>PLLERLKRRVVEGRKQGLEADLEEALKAGHKPLDLINGPLLAGMKEVGDLFGAGKMQLPFVLQAAEVMKRAVAYLEPHMEKKGEGKGTLVLATVKGDVHDIGKNLVDIILSNNGYRVVNLGIKVPIEEILKAVEAHKPHAVGMSGLLVKSTLVMKENLEYMRDRGYTLPVILGGAALTRSYVEELRAIYPNVYYAEDAFEGLRLMEELTGHAPPELTRKAPARPKREAPKVAPRARPVGEAPAVPRPPFFGVRVEEGLDLATIAHYVNKLALYRGQWGYSRKGLSREAWQALVEREAEPVFQRLLKEAMAEGWLEPKVLYGFFPVAREGEELLVFSPETGEVLERFRFPRQKGGGLSLVDYFRPRFAAPLGDEADWMPKEAFRAGARDVLGVQLVTMGEAPSRKAQALFASGAYQDYLFVHGFSVEMTEALAEYWHKRMRQMWGIAHQDATEIQKLFQQGYQGARYSFGYPACPDLADQAKLDRLMGFHRVGVRLTENFQLEPEHATSALVVHHPEARYFSVD[6x]

Cobalamin-dependent methionine synthase (MS) is a key enzyme in methionine and folate one-carbon metabolism. MS is a large multi-domain protein capable of binding and activating three substrates: homocysteine, folate, and S-adenosylmethionine for methylation. Achieving three chemically distinct methylations necessitates significant domain rearrangements to facilitate substrate access to the cobalamin cofactor at the right time. Here, we use a thermophilic MS homolog (tMS) as a functional MS model.

We selected cyanocobalamin (CN-Cbl), a stable and synthetic Cbl that does not support catalysis. To that end, apo-Cap:Cob:Act tMS crystals were soaked with CN-Cbl, yielding a structure of the holo-complex, solved to 2.95 Å resolution and one in the apo-form obtained prior to soaking, solved to 2.4 Å resolution. In the holo-Cap:Cob:Act structure, the Act domain remains positioned over the Cob domain, above the Cbl cofactor. Unexpectedly, the cofactor is found to bind in the His-off, base-off state. His761 forms a hydrogen bond with the phosphate tail of the DBI lower ligand, with the cobalamin bound in a His-off, base-off manner. Tyr1132 occludes the upper axial face of the Cbl cofactor, much like in previous reactivation structures captured in eMS and in contrast to our reported apo-tMS and apo-Cap:Cob:Act structures. There is minimal electron density in the upper axial position of the cofactor where the cyano group would reside, with a water molecule positioned 4.5 Å away from the cobalt center; this is in accord with previous reactivation conformation structures of MS. The absence of the cyano group indicates that the Co-CN bond is cleaved, likely via photoreduction during data collection. As such, the observation of Cbl binding in the His-off, base-off mode, without an axial ligand, was surprising and indicates that the captured Cbl is likely in the Co(II) state, and the cofactor was modeled as such. The requirement for reorganization of His761 and Tyr1132, in addition to the need for a reductive partner to reduce cob(II)alamin to cob(I)alamin, priming it for reactivation via methylation by SAM, indicates that the captured holo-structure is one en route to reactivation.> GSMSSERVLSYAPAFASALATSFFQELSRLKLDVLKLDSTCQPLTVNLDLHNIPKSADQVPLFLTNRSFEKHNNKRTNEVPLQGSIFNFNVLDEFKNLDKQLFLHQRALECWEDGIKDINKCVSFVIISFADLKKYRFYYWLGVPCFQRPSSTVLHVRPEPSLKGLFSKCQK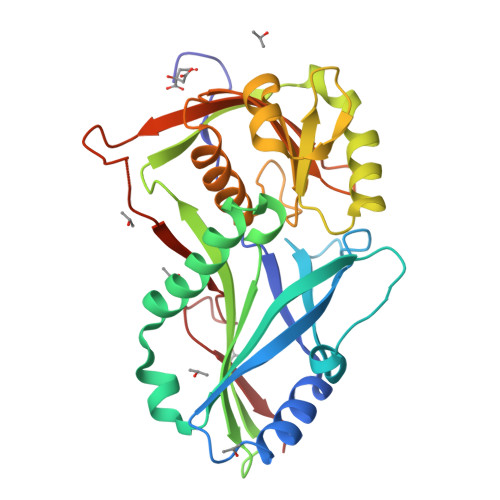WFDVNYSKWVCILDADDEIVNYDKCIIRKTKVLAIRDTSTMENVPSALTKNFLSVLQYDVPDLIDFKLLIIRQNEGSFALNATFASIDPQSSSSNPDMKVSGWERNVQGKLAPRVVDLS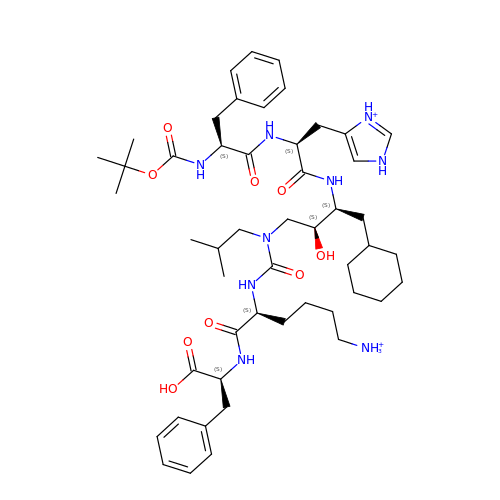6-ammonio-N-{[(2R,3R)-3-{[N-(tert-butoxycarbonyl)-L-phenylalanyl-3-(1H-imidazol-3-ium-4-yl)-L-alanyl]amino}-4-cyclohexyl-2-hydroxybutyl](2-methylpropyl)carbamoyl}-L-norleucyl-L-phenylalanine | C50 H77 N9 O9 | QBCYEBFUOBJJAC-KHVQSSSXSA-P> MVEPARKKQRIDRDTHHTVAEPVTEAKNTLYVSQLNEKINMQRLR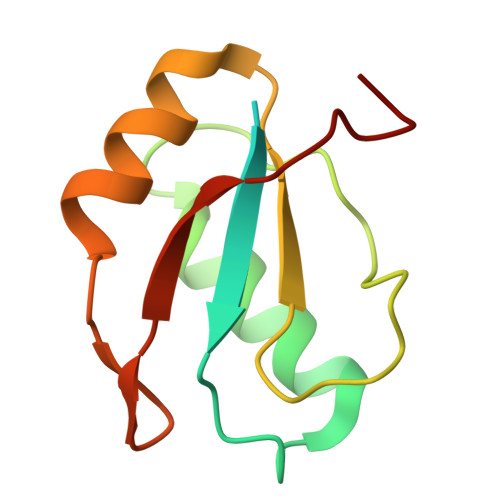VNLFLLFATFGEVLKVSMNFKKQRGQAFITMRTIDQASLAQISLNGERFFGKPLKVEFSKSETKTL>GADEEESTPCDNVETDQQTFACAAFNKQVAERELQSAYDELIERMRDQFGDEAGLMSRIEAAEKVWSQLRDADCKVETHAEQPGSNAYQIAWNSCIAQRSDERA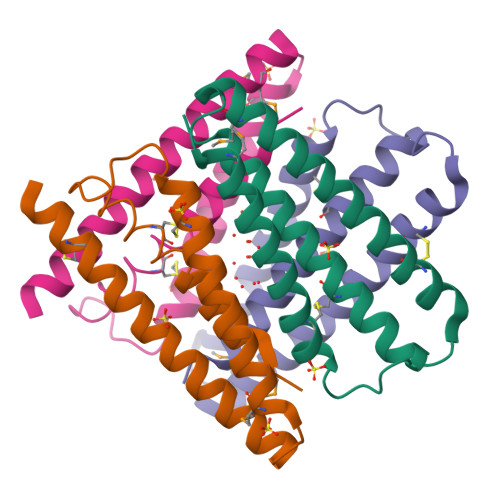EYLRSLGSQNSDEPAPED[2x]>SLDDHTRDPTVKAPDGNPSGWRTDGQWEHETLRRAVVHGVRLYNSGEFHESHDCFEDEWYNYGRGNTESKFLHGMVQVAAGAYKHFDFEDDDGMRSLFRTSLQYFRGVPNDYYGVDLLDVRTTVTNAL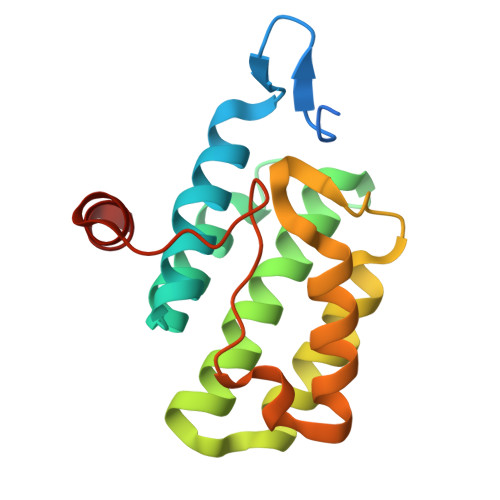SDPSALHGWQIRLDGEYPTCRPEDIEFAESLEH[2x]> MASSRCPAPRGCRCLPGASLAWLGTVLLLLADWVLLRTALPRIFSLLVPTALPLLRVWAVGLSRWAVLWLGACGVLRATVGSKSENAGAQGWLAALKPLAAALGLALPGLALFRELISWGAPGSADSTRLLHWGSHPTAFVVSYAAALPAAALWHKLGSLWVPGGQGGSGNPVRRLLGCLGSETRRLSLFLVLVVLSSLGEMAIPFFTGRLTDWILQDGSADTFTRNLTLMSILTIASAVLEFVGDGIYNNTMGHVHSHLQGEVFGAVLRQETEFFQQNQTGNIMSRVTEDTSTLSDSLSENLSLFLWYLVRGLCLLGIMLWGSVSLTMVTLITLPLLFLLPKKVGKWYQLLEVQVRESLAKSSQVAIEALSAMPTVRSFANEEGEAQKFREKLQEIKTLNQKEAVAYAVNSWTTSISGMLLKVGILYIG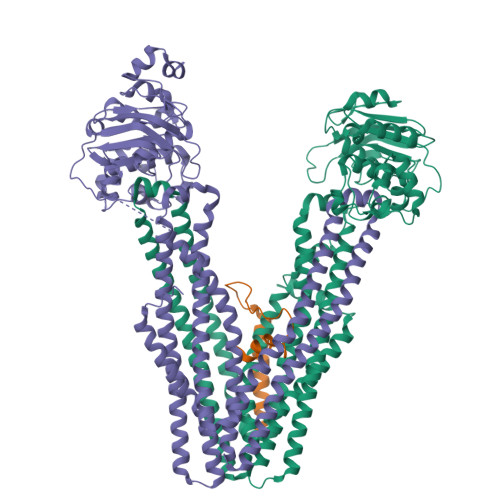GQLVTSGAVSSGNLVTFVLYQMQFTQAVEVLLSIYPRVQKAVGSSEKIFEYLDRTPRCPPSGLLTPLHLEGLVQFQDVSFAYPNRPDVLVLQGLTFTLRPGEVTALVGPNGSGKSTVAALLQNLYQPTGGQLLLDGKPLPQYEHRYLHRQVAAVGQEPQVFGRSLQENIAYGLTQKPTMEEITAAAVKSGAHSFISGLPQGYDTEVDEAGSQLSGGQRQAVALARALIRKPCVLILDDATSALDANSQLQVEQLLYESPERYSRSVLLITQHLSLVEQADHILFLEGGAIREGGTHQQLMEKKGCYWAMVQAPADAPESAQLEGSGGGAMVTTLSGLSGEQGPSGDMTTEEDSATHIKFSKRDEDGRELAGATMELRDSSGKTISTWISDGHVKDFYLYPGKYTFVETAAPDGYEVATPIEFTVNEDGQVTVDGEATEGDAHTSGGGHHHHHHHHHH;> MRLPDLRPWTSLLLVDAALLWLLQGPLGTLLPQGLPGLWLEGTLRLGGLWGLLKLRGLLGFVGTLLLPLCLATPLTVSLRALVAGASRAPPARVASAPWSWLLVGYGAAGLSWSLWAVLSPPGAQEKEQDQVNNKVLMWRLLKLSRPDLPLLVAAFFFLVLAVLGETLIPHYSGRVIDILGGDFDPHAFASAIFFMCLFSFGSSLSAGCRGGCFTYTMSRINLRIREQLFSSLLRQDLGFFQETKTGELNSRLSSDTTLMSNWLPLNANVLLRSLVKVVGLYGFMLSISPRLTLLSLLHMPFTIAAEKVYNTRHQEVLREIQDAVARAGQVVREAVGGLQTVRSFGAEEHEVCRYKEALEQCRQLYWRRDLERALYLLVRRVLHLGVQMLMLSCGLQQMQDGELTQGSLLSFMIYQESVGSYVQTLVYIYGDMLSNVGAAEKVFSYMDRQPNLPSPGTLAPTTLQGVVKFQDVSFAYPNRPDRPVLKGLTFTLRPGEVTALVGPNGSGKSTVAALLQNLYQPTGGQVLLDEKPISQYEHCYLHSQVVSVGQEPVLFSGSVRNNIAYGLQSCEDDKVMAAAQAAHADDFIQEMEHGIYTDVGEKGSQLAAGQKQRLAIARALVRDPRVLILDEATSALDVQCEQALQDWNSRGDRTVLVIAHRLQTVQRAHQILVLQEGKLQKLAQL;> GPTAAAAMGRGVPHIVMVDAYKRYKGGGSGGSGGGMVHVLERALLEQQSSACGLPGSSTETRPSHPCPEDPDVSRLRLLLVVLCVLFGLLCLLLI3-[6-azanyl-9-[(2~{R})-oxan-2-yl]purin-8-yl]prop-2-yn-1-ol | C13 H15 N5 O2 | 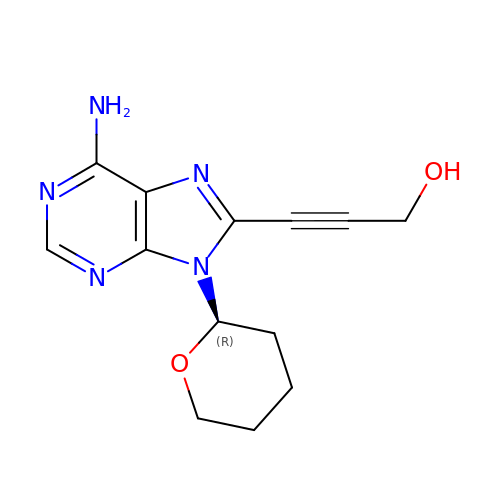AVGMEYBYAVAZNQ-SNVBAGLBSA-N>[8x]MVHYKLTYFAGRGLAEPIRQIFALAGQKYEDVRYTFQEWPKHKDEMPFGQIPVLEEDGKQLAQSFAIARYLSRKFGFAGKTPFEEALVDSVADQYKDYINEIRPYLRVVAGVDQGDPEKLFKELLLPAREKFFGFMKKFLEKSKSGYLVGDSVTYADLCLAEHTSGIAAKFPSIYDGFPEIKAHAEKVRSIPALKKWIETRPETKF

The structures of two major GSTs, Na-GST-1 and Na-GST-2 from Necator americanus, have been determined using recombinant protein expressed in and secreted by Pichia pastoris. GSTs are homodimers that catalyze the nucleophilic addition of reduced glutathione to various diverse electrophilic substrates consequently facilitating their inactivation, and extrusion. GSTs are a major detoxification system for helminths, which have limited detoxification enzymes and apparently lack the cytochrome P-450 dependent reactions. The fundamental/active units of both structures are homodimers with the classical GST topology of Nu class nematode specific GSTs.

Monoclinic Na-GST-2 contains an octamer in the asymmetric unit, corresponding to a Matthews' coefficient of 2.8 Å/Da and solvent content of 55%. The final refined monoclinic P21 model of Na-GST-2 indicates that differences in subunit structures prevent the higher order symmetry, and there are differences in side chain orientation across the monomers, and main chain residues; both termini; G-site vicinity (33–45); as well as in proximity to the dimerization domain (residues 101–156, 172–183) which are capable of breaking the higher order symmetry. Although no glutathione was added to the crystallization mixture, unambiguous density for a glutathione molecule was observed in G-site of each monomer of Na-GST-2. Apparently, Na-GST-2 usurps glutathione during the fermentation process. Our Na-GST-2 structure gives the first view of glutathione binding in a Nu class GST. Tyr 8 forms a hydrogen bond with the sulfur of glutathione. The side chain glutamyl residues of glutathione face the inter-domain cleft and are stabilized by hydrogen bonds with Trp 39. In addition, the glycyl residue in glutathione forms hydrogen bonds with Ser 64, while having an inter-molecular hydrogen bond from the conserved Asp 97 from across the dimer interface. As was observed in the structure of HpolGST, the H-site of Nu class GSTs as represented by Na-GST-2 forms a long, deep cleft. In the Na-GST-2 structure there are some ethylene glycol molecules from the cryoprotectant solution lining the surface of the H-site.>[4x]MPYDHNAEADFAASEVARMLVADPGLCYDAASLPASISASASYEPSAAGWPKADGLVSVLEGGTSTQRAIALEYKRPQEGIHGLLTAIGQAHGYLHKGYSGAAIVIPGRYSSHPTPAEYVRDVLNAISGSRAIAVFSYSPPDTTSPTPFAGRIQCVRPLVFDAGRVHLR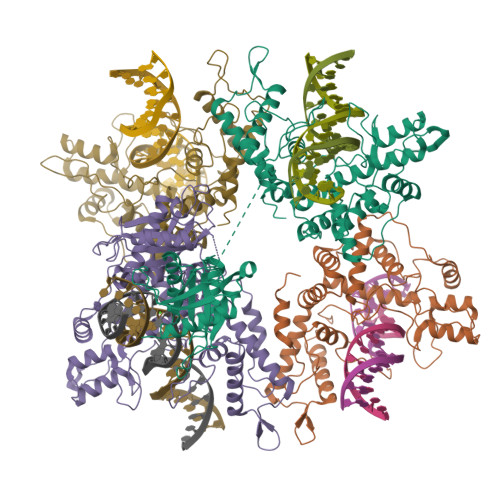PANQGPKTQWVHMREGSTTRDAFFRFLQVAKRLSADPTAPRPTLRSELVAAIGRLAPGRDPIEYITNTADNKFLTKVWQFFWLEWLATPAVLTPWKLEAGVYSAPGARTRILREDGTDFSQLWEGRVNSLKETIAGMLNRGEISEAQGWEAFVGGISATGGGQDKQGVRARAHSYREDIDSALAQLRWIEDDGLPTDQGYRFMTICERYGGANSRAAIDYMGATLIQTGRYASFLHYINRLSERKFAENPLAYTKPGPGGMPVFTEESYWEYLQDLETKLTDELRVMRKVSGRARPRVRTTFQVELTLLRNYGFVSSTRHRLGVGIPIDWEQVVQALNVDL> MSADSSPLVGSTPTGYGTLTIGTSIDPLSSSVSSVRLSGYCGSPWRVIGYHVVVWMMAGIPLLLFRWKPLWGVRLRLRPCNLAHAETLVIEIRDKEDSSWQLFTVQVQTEAIGEGSLEPSPQSQAEDGRSQAAVGAVPEGAWKDTALHKSEEAVSVGQKRVLRYYLFQGQRYIWIETQQAFYQVSLLDHGRSCDDVHRSRHGLSLQDQMVRKAIYGPNVISIPVKSYPQLLVDEALNPYYGFQAFSIALWLADHYYWYALCIFLISSISICLSLYKTRKQSQTLRDMVKLSMRVCVCRPGGEEEWVDSSELVPGDCLVLPQEGGLMPCDAALVAGECMVNESSLTGESIPVLKTALPEGLGPYCAETHRRHTLFCGTLILQARAYVGPHVLAVVTRTGFCTAKGGLVSSILHPRPINFKFYKHSMKFVAALSVLALLGTIYSIFILYRNRVPLNEIVIRALDLVTVVVPPALPAAMTVCTLYAQSRLRRQGIFCIHPLRINLGGKLQLVCFDKTGTLTEDGLDVMGVVPLKGQAFLPLVPEPRRLPVGPLLRALATCHALSRLQDTPVGDPMDLKMVESTGPQLQAMEEPPVPVSVLHRFPFSSALQRMSVVVAWPGATQPEAYVKGSPELVAGLCNPETVPTDFAQMLQSYTAAGYRVVALASKPLPTVPSLEAAQQLTRDTVEGDLSLLGLLVMRNLLKPQTTPVIQALRRTRIRAVMVTGDNLQTAVTVARGCGMVAPQEHLIIVHATGQPASLEFLPMESPTAVNGVKDPDQAASYTVEPDPRSRHLALSGPTFGIIVKHFPKLLPKVLVQGTVFARMAPEQKTELVCELQKLQYCVGMCGDGANDCGALKAADVGISLSQAEASVVSPFTSSMASIECVPMVIREGRCSLDTSFSVFKYMALYSLTQFISVLILYTINTNLGDLQFLAIDLVITTTVAVLMSRTGPALVLGRVRPPGALLSVPVLSSLLLQMVLVTGVQLGGYFLTLAQPWFVPLNRTVAAPDNLPNYENTVVFSLSSFQYLILAAAVSKGAPFRRPLYTNVPFLVALALLSSVLVGLVLVPGLLQGPLALRNITDTGFKLLLLGLVTLNFVGAFMLESVLDQCLPACLRRLRPKRASKKRFKQLERELAEQPWPPLPAGPLR

ATP13A2 belongs to the orphan P5B adenosine triphosphatases (ATPase) family and has been established as a lysosomal polyamine exporter to maintain the normal function of lysosomes and mitochondria. Here, using single-particle cryo-EM, we present the structures of full-length human ATP13A2 in three distinct conformations including an E1 state (apo), an E1P-ADP state with ATP and Mg2+, and an E2-Pi state with SPM, phosphatidic acid (PA), and phosphatidylinositol(3,5)bisphosphate [PI(3,5)P2]. The structure of the human ATP13A2 adopts the typical P-type ATPase fold with overall dimensions of 125 Å × 75 Å × 70 Å, including ten transmembrane (TM) helices and three conserved cytoplasmic domains [N (nucleotide-binding) domain; A (actuator) domain; and P (phosphorylation) domain]. In addition, the P5B type ATP13A2 also comprises two specific domains: a C-terminal extension domain (CTD) laying close to the P-domain and an N-terminal domain (NTD) preceding the A domain showing amphipathic feature.

The purified human ATP13A2 was subjected to cryo-EM analysis under three different conditions, apo state, E1P-ADP state (with Mg2+, ATP, and SPM), and E2-Pi state [with PI(3,5)P2, PA, and SPM], and at overall resolutions of 3.3, 3.0, and 3.6 Å, respectively. The E1P-ADP state map showed well-resolved densities to allow confident de novo model building for most of the protein regions, the other two state models were reconstructed according to the E1P-ADP state structure. To describe the overall architecture and the specific domains, we will reference the 3.0-Å-resolution E1P-ADP state structure because the flexible cytosolic domains are better resolved in this map. ATP binds to ATP13A2 and the resultant phosphoryl transfer reaction induces the rearrangement of the N domain, by which the N domain tilt around 30° to lay close to the A and P domain, thus sealing the crevice formed by the N and P domain compared to the E1 state. After the E1-ATP-to-E1P-ADP transition, ADP molecular was stabilized by several polar interactions, in which the adenine ring of the ADP forms interaction with F630 from the N domain via π–π interaction, whereas the phosphate group of ADP interacts with the neighboring N881, K859, D882, and T515 from the P domain via hydrogen-bonds interactions. In addition, two Mg2+ ions were coordinated by the carbonyl of T515 and phosphorylated D513. Mutagenesis of the aspartate (D513A) resulted in a reduced activity compared with wild-type proteins, highlighting the essential role of this conserved aspartate in ATP13A2 activity. The C terminal helix interacts with the neighboring P domain via several interactions, including the hydrogen-bonds interactions via P1172-R821, E1165-K843, F1159-L869, and K1157-Q508.>MTDKKIVLYSLTTCGFCQAIKKMFDDLAVGHLCIQADELTGEEKKQALRDLRKVNPKCSFPTVVIDETVVVGPKIQEIKEKIGIRTEVDELYEVLKKKNEPKGYYLNGDREKTFELIRGLLTNKKRYGYMACPCRLASGDRNNDRDIICPCLYREPDVKEFGSCYCTLYVSADWY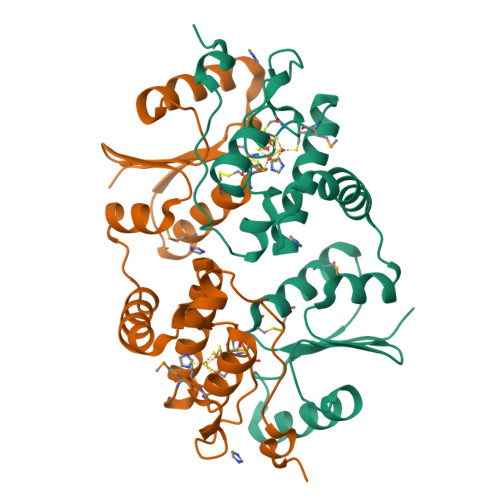TGKIERQEVAERRPPEHYELD[2x]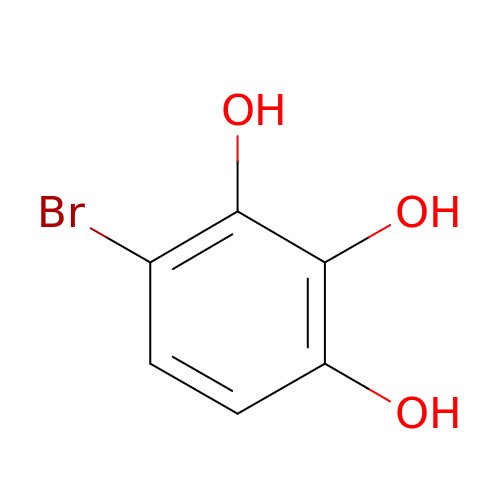4-bromobenzene-1,2,3-triol | C6 H5 Br O3 | TYRFQQZIVRBJAK-UHFFFAOYSA-N>[4x]GPHMTGLAAISDALAADLAGLSFSSPVAHV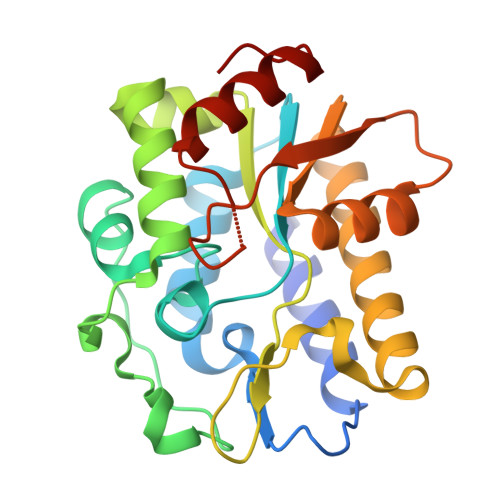YNPLLYAREPHVAYLSRFGSPPKEVLFVGMNPGPWGMAQTGVPFGEVAVVTEWLGINGTVTRPAGEHPKKRVDGFACRRSEVSGRRLWGFIRERFGTPERFFARFFVANYCPLLFLTAEGGNITPDKLRRGEQEPLFAACDLALRRTVVLLRPRVVIGVGAFAEARCHEALEGFDVEVGRIIHPSPASPAANRDWAGTALRQLAELGVDF Tripartite α-PFTs are members of the ClyA α-PFT family. Proteins in this family undergo a large scale conformational change from a compact soluble structure, where the hydrophobic residues are hidden often within a β-tongue motif, to an extended pore structure with the hydrophobic residues exposed in two extended α-helices which insert into the cell membrane. Here we show that S. marcescens has a tripartite haemolytic α-PFT (SmhABC), and propose a mechanism of pore assembly. We present the structures of the soluble A component (SmhA), as well as the soluble and pore conformations of the B component (SmhB).

As expected, soluble SmhB folds into the family observed β-tongue structure, with a five-helix bundle tail (α1, α2, α3, α6, α7), and a head domain containing three α-helices (α4, α5, α8) alongside a four-strand β-sheet (β1, β2, β3, β4), which includes the β-tongue motif (β1 and β2). The head domain of SmhB is largely hydrophobic. This is particularly evident in the β-tongue and helices α4 and α5, which together constitute the predicted hydrophobic transmembrane region (G175—L233). The crystal asymmetric unit contained two closely related monomeric AhlB molecules (RMSD Cα 0.56 Å) with the only significant differences in the tail domain, where α7 from chain A folds as a single helix with a kink at S320, while in chain B α7 is divided into α7a and α7b by a short loop region (T319-V321). AhlB and SmhB use both a short β-strand and a short helix connected by a loop, while SmhA uses only a short loop perpendicular to β1. The second region is between the N-terminus and β-tongue, which includes a family conserved glutamine (Q38 SmhA, Q32 SmhB, Q45 NheA) on the N-terminal helix α1 that forms hydrogen bonds with the β-sheet backbone of the β-tongue. In addition, both SmhA and SmhB contain a family conserved (conserved in all but 1 sequence) lysine residue at the C-terminus (K333 in both SmhA and SmhB) that forms a hydrogen bond with a conserved hydroxyl (T81 SmhA; T78 SmhB) on helix α2. As the overall structures of the soluble and pore forms of SmhB are almost identical to those of AhlB (RMSD Cα 0.64 Å and 0.46 Å, respectively),, not surprising given the high level of sequence identity (62%), we investigated if these structural similarities also conveyed functional similarities. The B and C components interact at a binding interface located around residues 95–123 of SmhB, this could break latches 1 and 2 on the B component, releasing the β-tongue, C-terminus, and N-terminus to initiate the transformation into the B component pore conformation.

>MTIPTLYMNDGMNAQSSQALHIQTYCNSVRQQIPVDFGRFPNLRESERQINTGLGAARQHAEHYLKDIQPLIIRNVTNIQDYFETQNLISTVMPSGATKEQWLSALGMVSDKAKEYQEVSANTRRTIGSLNDKLIIDSNNYQLIVVNLNNVVNGNNGVLEQLNRDIDGINAAIDGAIAGIVVGGLLVIGGAIVTAIGAVAGLVTAGTSTPVVMGGIAMMTAGAGGVIGGAIVLDKSLSAREKLYRDRSQLNSEVLVASQIGSGYRGLQTQAQSAVTAATQMNNAWDSLTSELETLNANLRKGIIDDSFLRQLFLTASQTSVTKVLDGTKIIKQQMAGVVVREVPANQSIADFVKRLAALEHHHHHH[2x]>MGFLSGKRILVTGVASKLS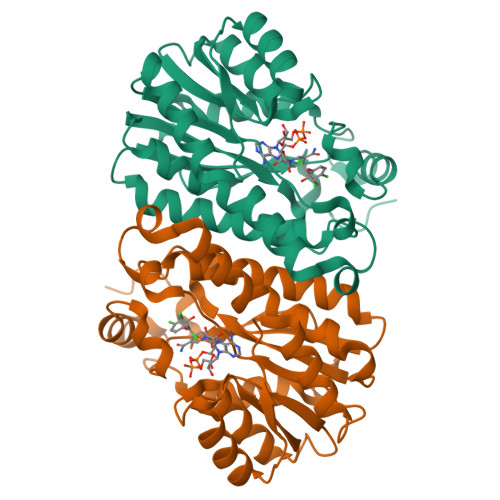IAYGIAQAMHREGAELAFTYQNDKLKGRVEEFAAQLGSDIVLQCDVAEDASIDTMFAELGKVWPKFDGFVHSIAFAPGDQLDGDYVNAVTREGFKIAHDISSYSFVAMAKACRSMLNPGSALLTLSYLGAERAIPNYNVMGLAKASLEANVRYMANAMGPEGVRVNAISAGPIRTLAASGIKDFRKMLAHCEAVTPIRRTVTIEDVGNSAAFLCSDLSAGISGEVVHVDGGFSIAAMNELELKLEHHHHHH[2x]> GMEYVEALYQFDPQQDGDLGLKPGDKVQLLEKLSPEWYKGSCNGRTGIFPANYVKPA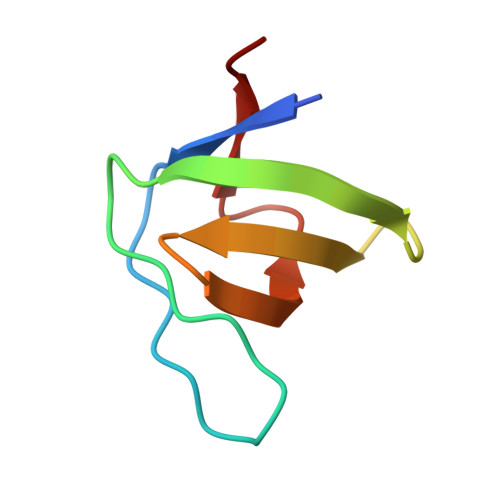F> SNAMNITLLKSKIHRASVTEARLDYIG;> XISIDEKLLQASGILEYEKVQVVNVNNGAR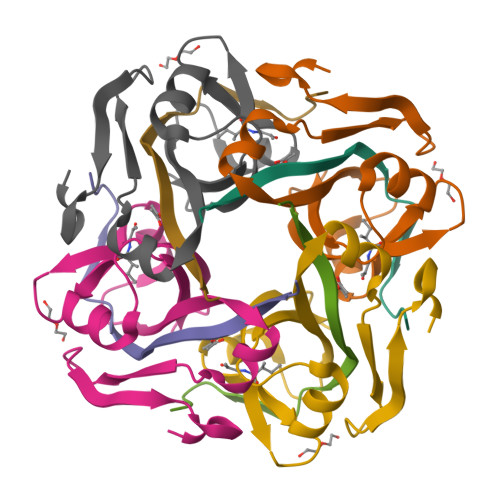FETYTIATQEEGVVCLNGAAARLAEVGDKVIIMSYADFNEEEAKTFKPKVVFVDENNTATKITNYEKHGAIF>[2x]TLLGTALRPAATRVMLLGSGELGKEVAIECQRLGVEVIAVDRYADAPAMHVAHRSHVINMLDGDALRRVVELEKPHYIVPEIEAIATDMLIQLEEEGLNVVPCARATKLTMNREGIRRLAAEELQLPTSTYRFADSESLFRE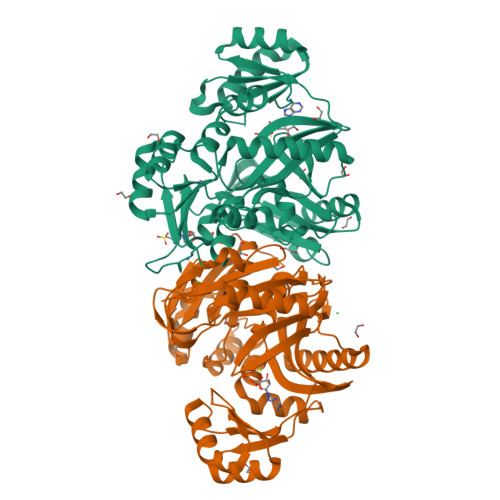AVADIGYPCIVKPVMSSSGKGQTFIRSAEQLAQAWKYAQQGGRAGAGRVIVEGVVKFDFEITLLTVSAVDGVHFCAPVGHRQEDGDYRESWQPQQMSPLALERAQEIARKVVLALGGYGLFGVELFVCGDEVIFSEVSPRPHDTGMVTLISQDLSEFALHVRAFLGLPVGGIRQYGPAASAVILPQLTSQNVTFDNVQNAVGADLQIRLFGKPEIDGSRRLGVALATAESVVDAIERAKHAAGQVKVQG>SATETQIRIGVMGCADIARKVSRAIHLAPNATISGVASRSLEKAKAFATANNYPESTKIHGSYESLLEDPEIDALYVPLPTSLHVEWAIKAAEKGKHILLEKPVAMNVTEFDKIVDACEANGVQIMDGTMWVHNPRTALLKEFLSDSERFGQLKTVQSCFSFAGDEDFLKNDIRVKPGLDGLGALGDAGWYAIRATLLANNFELPKTVTAFPGAVLNEAGVILSCGASLSWEDGRTATIYCSFLANLTMEITAIGTKGTLRVHDFIIPYKETEASFTTSTKAWFNDLVTAWVSPPSEHTVKTELPQEACMVREFARLVGEIKNNGAKPDGYWPSISRKTQLVVDAVKESVDKNYQQI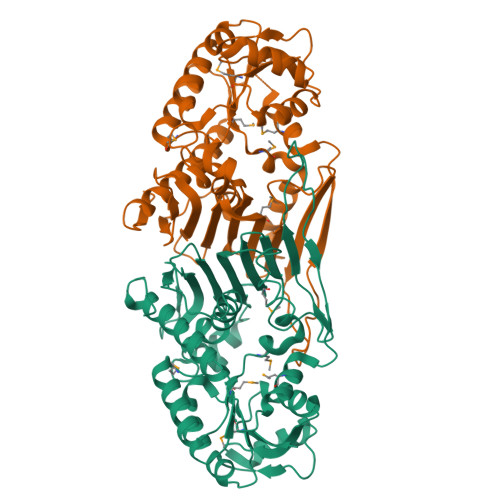SLSGR[2x]>GPGGVEALEDALAQIKSVNNALQERVEAVAADVRTFSEGYIKAIEEHRDKLLQQLDDIRIQRETA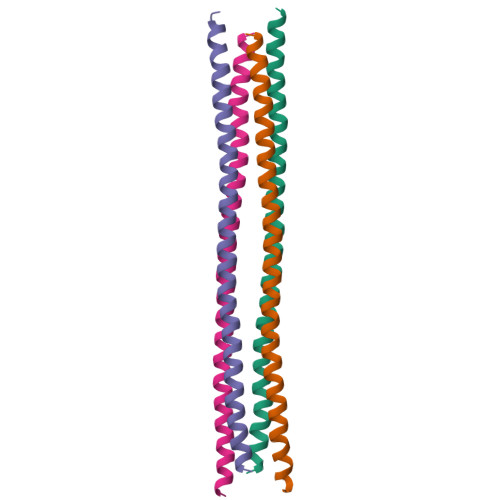LQLQKAQLEQLLADMRTGVE[4x]(2~{S})-3-methyl-2-[pentanoyl-[[4-[2-(2~{H}-1,2,3,4-tetrazol-5-yl)phenyl]phenyl]methyl]amino]butanoic acid | C24 H29 N5 O3 | 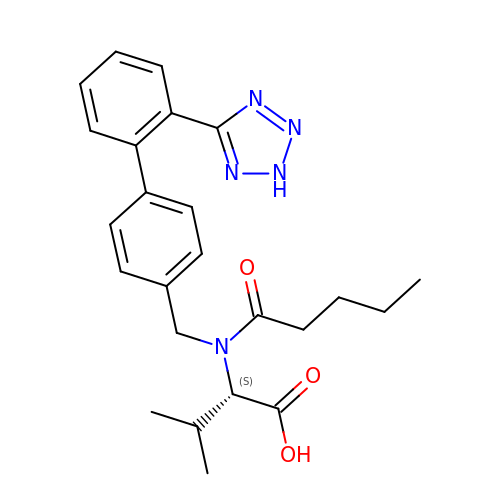ACWBQPMHZXGDFX-QFIPXVFZSA-N The two recently opened beamlines for macromolecular crystallography at NSLS-II have launched the microcrystallography field into new territory, with flux densities up to two orders of magnitude brighter than those previously available. In this study, we highlight the capabilities of the AMX and FMX beamlines at NSLS-II by describing structure determination from single crystal vector data collection and two methods for multicrystal data collection. The advent of next generation synchrotron beamlines has necessitated the development of new strategies to fully benefit from the increased beam intensity and smaller beam sizes while minimizing radiation damage. The high dose rates, in conjunction with the newly developed ultrafast raster scanning goniometer brings formerly time-consuming serial crystallography measurements into the minutes range. These new opportunities mean that inhomogeneous large crystals can now deliver high quality data collected from their best volume, and crystals as small as 5 to 10 µm can deliver one or more complete datasets.

B. cereus CDP-Chase is a member of the Nudix hydrolase superfamily, which are a family of enzymes that hydrolyze nucleoside diphosphates linked to some other moiety, x. It is a bifunctional enzyme that can hydrolyze CDP-choline with the typical nudix reaction in addition to a non-nudix exonuclease reaction on RNA. Although its endogenous substrate is CDP-choline, CDP-Chase can also hydrolyze other nudix substrates including ADP-ribose. Data for the B. cereus CDP-Choline Pyrophosphatase (CDP-Chase) crystals were collected on a larger, single crystal (60 × 30 × 20 µm) using vector collection, and the smaller crystals were used for a multicrystal approach for direct comparison (see Section 2.2.1). For the single crystal, the data were indexed, integrated, and scaled with FastDP to a resolution of 2.08 Å with 〈I/σ(I)〉 of 2.6. Cocrystals grown in the presence of ADP-ribose, a suboptimal substrate for CDP-Chase, do not show electron density for the complete substrate molecule or the expected product of hydrolysis, phosphoribose. Electron density observed in the active site was consistent with separate ribose and phosphate molecules. The ribose was bound directly by B-R31 and formed water-mediated interactions with B-W98 and A-Y22. When cocrystallized with ADP-ribose, loops A&B 86-91 and B159-164 become ordered, while the loop B133-142 becomes disordered. Overall, the ordering of previously disordered loops and the sizable changes in the conformations of other key catalytic loops suggests that these crystals have captured another catalytically relevant snapshot of CDP-Chase, most likely the active conformation.

>MTIKWIDWVKQIQSIAQAGLTYSKDVYDIERFQQLRDISISMMSHYTKTDWEVVEKLFASETGYQTPKVDIRAVVFQNEKLLFVKEKSDGKWALPGGWADVGYTPTEVAAKEVFEETGYEVDHFKLLAIFDKEKHQPSPSATHVYKIFIGCEIIGGEKKTSIETEEVEFFGENELPNLSIARNTEDQIKEMFAYMKDPQKEKLID[2x]>[4x]XGEIQKQLKEI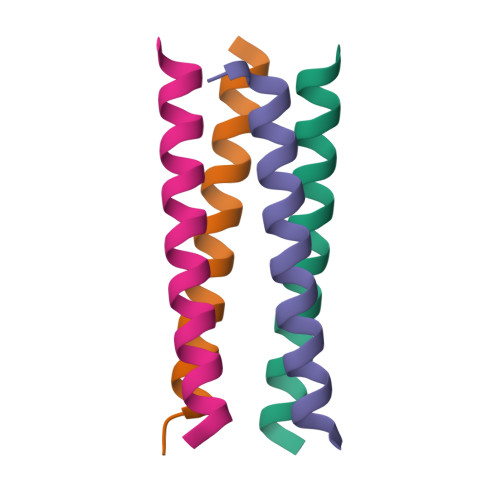QKQLKEIQWQLKEIQKQLKGX> MEEQPQMQDADEPADSGGEGRAGGPPQVAGAQAACSEDRMTLLLRLRAQTKQQLLEYKSMVDASEEKTPEQIMQEKQIEAKIEDLENEIEEVKVAFEIKKLALDRMRLSTALKKNLEKISRQSSVLMDNMKHLLELNKLIMKSQQESWDLEEKLLDIRKKRLQLKQASESKLLEIQTEKNKQKIDLDSMENSERIKIIRQNLQMEIKITTVIQHVFQNLILGSKVN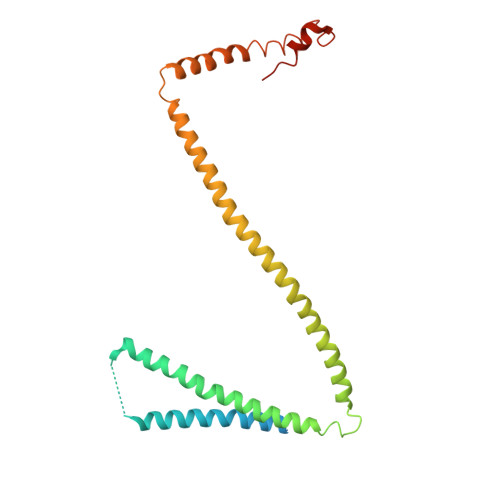WAEDPALKEIVLQLEKNVDMM> MANFVIPYLKPVADFWNSLCIDQHQDSLFQFKGQTGSLGTDWTSKYLRSEQDVYNHKYLQYHKRVHEAPELTDVISDNVYRLTLFAGVERVLSVRQAQAILKTQFAGATENISGAFQTVLNGGIFRRGYFRGALLNLLQFCGAPYQSLIWSRNSGIT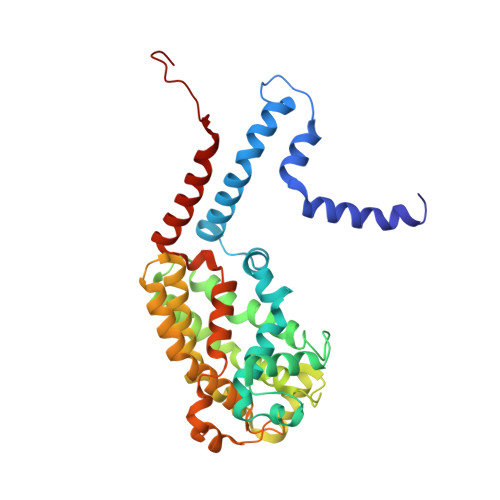NQVIVSSIFEAFFYPLDTVKTLIYNDVQGKYKGAFHCASQVVQNAGWSRLYAGIFQKLIFNSALIFHLNQVWDGSSQQWASLALVAAAYPLLVLKTRFQVAGTPLALATSNEVLKVNRKTLYAGLVPYLIFNTLFAYEFAAWHSSTAQERVIGGLQNAMKQFSSPAAEQVWSS>MDYKDDDDKEPGGARLRLQRTGGLGGERERQPCGDGNTETHRAPDLVQWTRHMEAVKAQLLEQAQGQLRELLDRAMREAIQSYPSQDKPLPPPPPGSLSRTQEPSLGKQKVFIIRKSLLDELMEVQHFRTIYHMFIAGLCVFIISTLAIDFIDEGRLLLEFDLLIFSFGQLPLALVTWVPMFLSTLLAPYQALRLW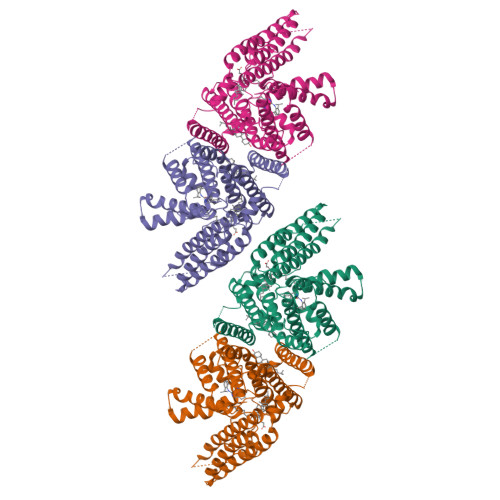ARGTWTQATGLGCALLAAHAVVLCALPVHVAVEHQLPPASRCVLVFEQVRFLMKSYSFLREAVPGILRARRGEGIQAPSFSSYLYFLFCPTLIYRETYPRTPYVRWNYVAKNFAQALGCVLYACFILGRLCVPVFANMSREPFSTRALVLSILHATLPGIFMLLLIFFAFLHCWLNAFAEMLRFGDRMFYRDWWNSTSFSNYYRTWNVVVHDWLYSYVYQDGLRLLGARARGVAMLGVFLVSAVAHEYIFCFVLGFFYPVMLILFLVIGGMLNFMMHDQRTGPAWNVLMWTMLFLGQGIQVSLYCQEWYARRHCPLPQATFWGLVTPRSWSCHT[4x]>[2x]MRGSHHHHHHGSRTYSD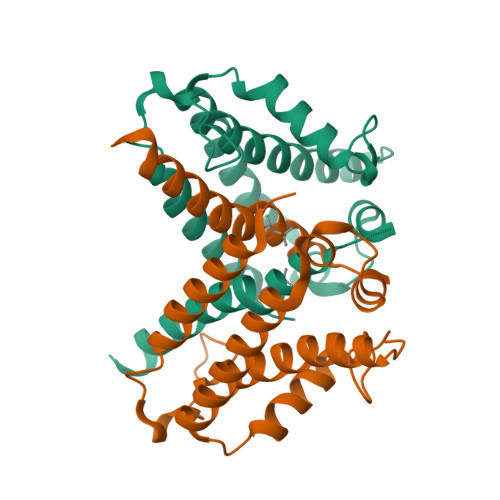KNELKEEVLKSYKKYIAEFNDIPEKLKDLRIDEVDRTPAENLAYQVGWTTLILKWESDEQSGLEVKTPTETFKWNQLGELYQHFTETYASLTIKELTAQLNDNVDAIGNMIDSMSDEVLFKPHMRNWADSATKNAVWEVYKFIHINTVAPFGTFRTKIRKWKKVALK>MSEAQPDARSDARDLTAFQKNILTVLGEEARYGLAIKRELEEYYGEEVNH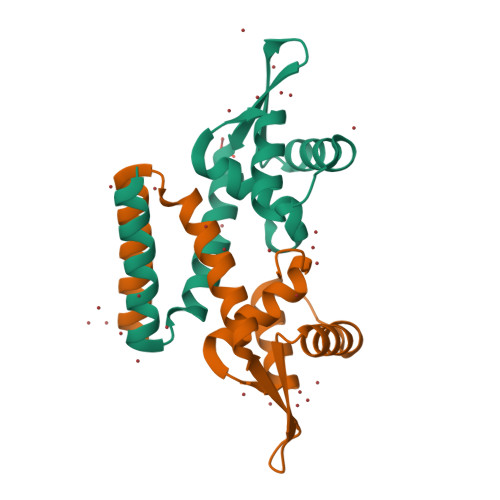GRLYPNLDDLVNKGLVEKSELDKRTNEYALTNEGFDAVVDDLEWTLSKFVADADRRERVETIVADDAAALEHHHHHH[2x]>[2x]ENLKLGFLVAQPEEPASQTQWKFADKAGKDLGFEVIKIAV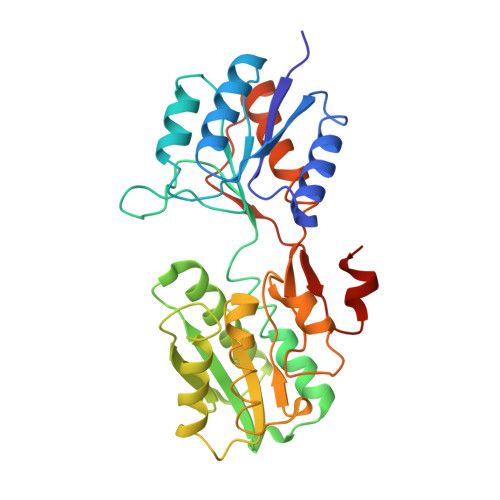PDGEKTLNAIDSLAASGAKGFVISTPDPKLGSAIVAKARGYDMKVIAVDNQFVNAKGKPMDTVPLVMEAATKIGERQGQELYKEMQKRGWDVKESAVMAITANELDTARRRTTGSMDALKAAGFPEKQIYQVPTKSEDIPGAFDAANSMLVQHPEVKHWLIVGMNDSTVLGGVRATEGQGFKAADIIGIGINGVDAVSELSKAQATGFYGSLLPSPDVHGYKSSEMLYNWVAKDVEPPKFTEVTDVVLITRDNFKEECEKKGLGGK> MDGSGEQLGSGGPTSSEQIMKTGAFLLQGFIQDRAGRMAGETPELTLEQPP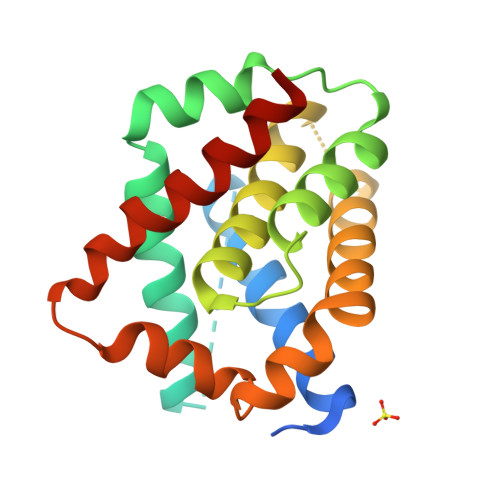QDASTKKLSESLRRIGDELDSNMELQRMIADVDTDSPREVFFRVAADMFADGNFNWGRVVALFYFASKLVLKALSTKVPELIRTIMGWTLDFLRERLLVWIQDQGGWEGLLSYFGTPTWQTVTIFVAGVLTASLTIWKKMG> GSMSRSKRDNNFYSVEIGDSTFTVLKRYQNLKPIGSGAQGIVCAAYDAILERNVAIKKLSRPFQNQTHAKRAYRELVLMKCVNHKNIIGLLNV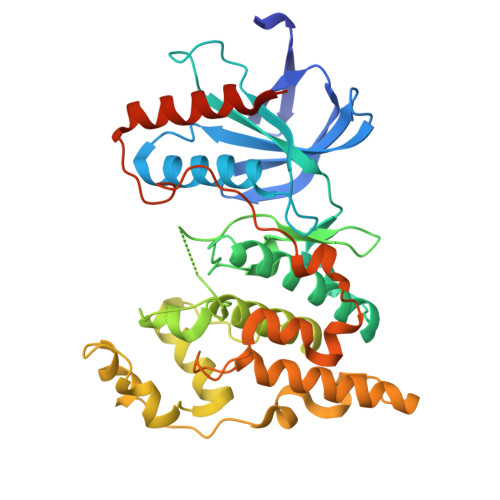FTPQKSLEEFQDVYIVMELMDANLCQVIQMELDHERMSYLLYQMLCGIKHLHSAGIIHRDLKPSNIVVKSDCTLKILDFGLARTAGTSFMMVPFVVTRYYRAPEVILGMGYKENVDIWSVGCIMGEMIKGGVLFPGTDHIDQWNKVIEQLGTPCPEFMKKLQPTVRTYVENRPKYAGYSFEKLFPDVLFPADSEHNKLKASQARDLLSKMLVIDASKRISVDEALQHPYINVWYDPSEAEAPPPKIPDKQLDEREHTIEEWKELIYKEVMDLEERTKNGVIRGQPSPLAQVQQ7-(difluoromethoxy)-N-[trans-4-(2-hydroxypropan-2-yl)cyclohexyl]quinoline-3-carboxamide | C20 H24 F2 N2 O3 | 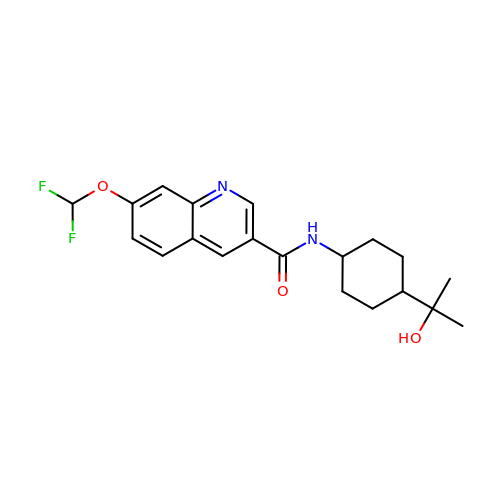YRWMWDLEUYLURJ-SHTZXODSSA-N>MRGSHHHHHHGSKFCRFGQRGQEKPGIIDADGNIRDLSGVVPELTIDALAAAKGADIALLPLVEGEPRYGVPVKGIGKIVAIGLNYEDHAIESNLPIPTEPMMFMKALSSLNGPNDEVVLPKNSTHGDWEVELGVVIGETCRFVSEDEALSKVAGYVLVNDVSERFNQKQRGTQWSKGKGHDTFCPVGPWLVTPDEVGDPQDLDVHLDVNGERMQTGNTKTMIFNVAQLISYV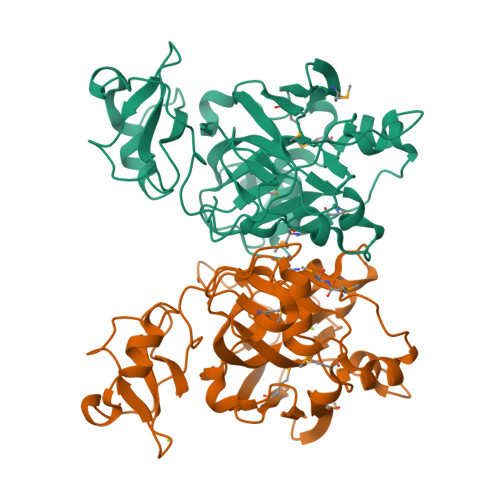SEYITLYPGDLMITGTPPGVGEGKKPQAIYLKAGDVMELGIEKLGTQRQQVSEWRHLGDEVFG[4x]> HAT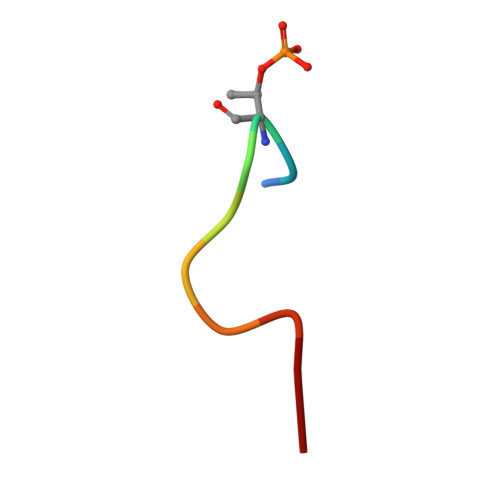PPKKEAD Ski7 is a cofactor of the cytoplasmic exosome in budding yeast, functioning in both mRNA turnover and non-stop decay (NSD), a surveillance pathway that degrades faulty mRNAs lacking a stop codon. The C-terminal region of Ski7 (Ski7C) shares overall sequence similarity with the translational GTPase (trGTPase) Hbs1, but whether Ski7 has retained the properties of a trGTPase is unclear. Ski7C is organized in three domains. However, a suboptimal polar residue at the putative catalytic site and an unusual polar residue that interacts with the γ-phosphate of GTP distinguish Ski7 from other trGTPases, suggesting it might function rather as a GTP-binding protein than as a GTP-hydrolyzing enzyme.

We obtained crystals of Ski7C in the presence of GDP and magnesium ions using inorganic phosphate as precipitating agent. We solved the structure with a selenomethionine-based single-wavelength anomalous dispersion experiment and refined it at 2.2-Å resolution to Rfree of 24.6%, Rwork of 21.7%, and good stereochemistry. The refined structure (referred to as Ski7C-GDP-Pi) includes most of the Ski7C polypeptide chain (with the exception of short disordered loop regions) and also includes GDP, a molecule of inorganic phosphate (Pi) and an Mg2+ ion. Manganese was soaked into the crystal prior to data collection to substitute Mg2+ and to unambiguously identify the position of the divalent cation in the electron density using anomalous scattering. In Ski7C-GDP-Pi, the inorganic phosphate is clearly separated from the β-phosphate of the GDP (with a phosphate-phosphate distance of 4.2 Å). The γ-phosphate of the GTP-bound structure and the inorganic phosphate of the GDP-Pi-bound structure are adjacent to each other, but they do not coincide. In the case of the Ski7C-GDP-Pi structure, the complex either mimics a putative post-hydrolysis state (e.g. before release of the Pi product and conversion to an inactive GDP-bound state) or engages the small molecules supplied at high concentrations with the crystallization buffer (i.e. GDP and inorganic phosphate) to mimic a GTP-bound state. Except for a loop approaching the sugar moiety of the nucleotide that is involved in a crystal contact in the Ski7C-GDP-Pi crystal, the structure of Ski7C is essentially identical in the Ski7C-GDP-Pi and Ski7C-GTP complexes, superposing with a root-mean-square deviation of 0.53 Å over all atoms. The work we report here indicates that the C-terminal G domain of S. cerevisiae Ski7 possesses the structural features of a canonical trGTPase not only in terms of domain structure, as expected from sequence analysis, but also in terms of conformation. Both the GTP-bound and the GDP-Pi-bound complexes of Ski7C adopt the conformation typical of trGTPases in the active GTP-bound state and show an overall similar nucleotide-binding pocket.

> GPDSMSIDIHSFIATHPLNLTCLFLGDTNAGKSTLLGHLLYDLNEISMSSMRELQKKSSNLDPSSSNSFKVILDNTKTERENGFSMFKKVIQVENDLLPPSSTLTLIDTPGSIKYFNKETLNSILTFDPEVYVLVIDCNYDSWEKSLDGPNNQIYEILKVISYLNKNSACKKHLIILLNKADLISWDKHRLEMIQSELNYVLKENFQWTDAEFQFIPCSGLLGSNLNKTENITKSKYKSEFDSINYVPEWYEGPTFFSQLYLLVEHNMNKIETTLEEPFVGTILQSSVLQPIAEINYVSLKVLINSGYIQSGQTIEIHTQYEDFHYYGIVSRMKNSKQILETNTKNNISVGLNPDILEVLVKIHNTEDFTKKQFHIRKGDIIIHSRKTNTLSPNLPNTLKLLALRLIKLSIQTHALSDPVDLGSELLLYHNLTHNAVKLVKILGTNDISINPNQSLIVEVEIIEPDFALNVIDSKYITNNIVLTSIDHKVIAVGRIACQ(5R)-5-[(4-fluorophenyl)methyl]-5-(2-hydroxyethyl)-3-(2-methoxyethyl)imidazolidine-2,4-dione | C15 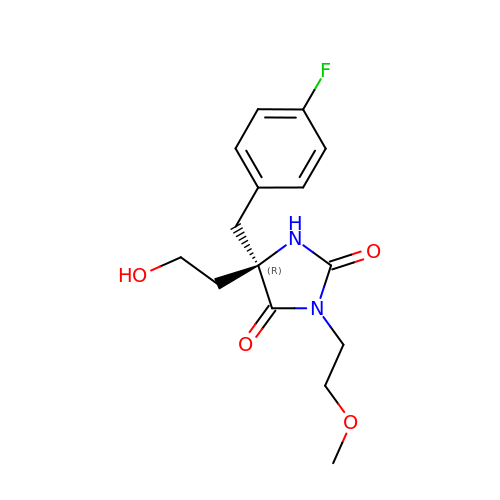H19 F N2 O4 | LEFBUGONDDVZFX-HNNXBMFYSA-N> GHMALSSLNIIHIAAPHLEALNIATGETINFSSREDDHAILIYKLEPTTGMLRTRAYIGQHMPL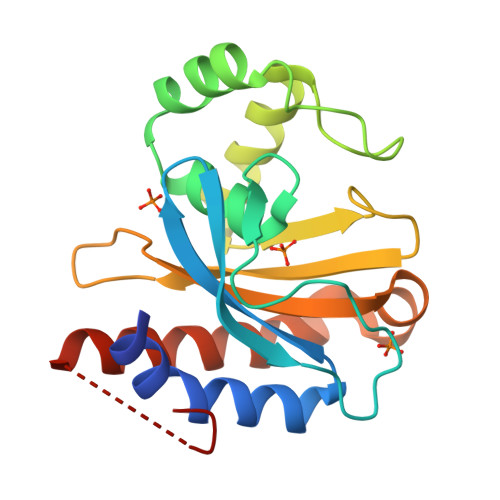YCSAMGKIYMAFGHPDYVKSYWESHQHEIQPLTRNTITELPAMFDELAHIRESGAAMDREENELGVSCIAVPVFDIHGRVPYAVSISLSTSRLKQVGEKNLLKPLRETAQAISNELGFTVRDDLGAITG>MKLLLLLLCLGLTLVCG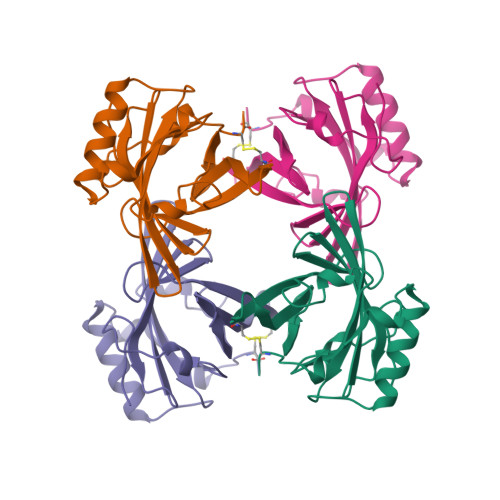HAEEASSTRGNLDVAKLNGDWFSIVVASNKREKIEENGSMRVFMQHIDVLENSLGFKFRIKENGECRELYLVAYKTPEDGEYFVEYDGGNTFTILKTDYDRYVMFHLINFKNGETFQLMVLYGRTKDLSSDIKEKFAKLCEAHGITRDNIIDLTKTDRCLQARG[4x]>[4x]MEKTTTQELLAQAEKICAQRNVRLTPQR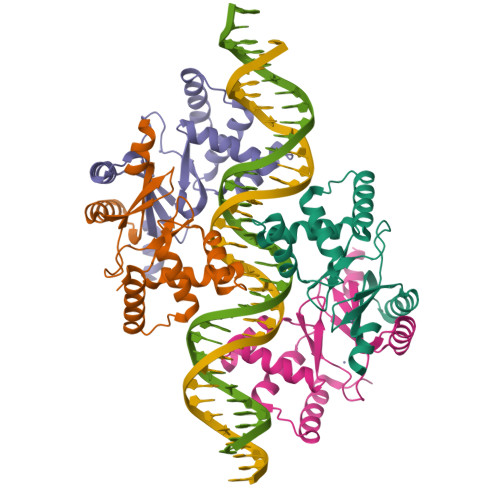LEVLRLMSLQDGAISAYDLLDLLREAEPQAKPPTVYRALDFLLEQGFVHKVESTNSYVLCHLFDQPTHTSAMFICDRCGAVKEECAEGVEDIMHTLAAKMGFALRHNVIEAHGLCAACVEVEACRHPEQCQHDHSVQVKKKPR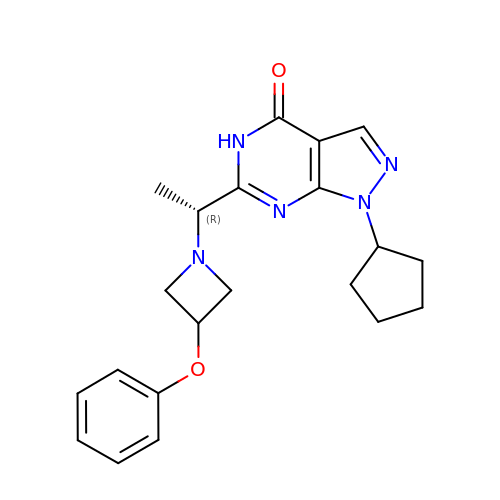1-cyclopentyl-6-[(1R)-1-(3-phenoxyazetidin-1-yl)ethyl]-1,5-dihydro-4H-pyrazolo[3,4-d]pyrimidin-4-one | C21 H25 N5 O2 | KKFKLLKJGDFZBA-CQSZACIVSA-N>[4x]MSQNQVPKWIQLNNEIMIQKDGKFQFDKDKEAVHSYFVDYINQNTVFFHNLKEKLDYLVENQYYEEEFLSLYSFEDIKEVFKTAYAKKFRFPSFMSAFKFYNDYALKTNDKKKILERYEDRISIVALFFANGDTEKAKEYVNLMINQEYQPSTPTFLNAGRKRRGEL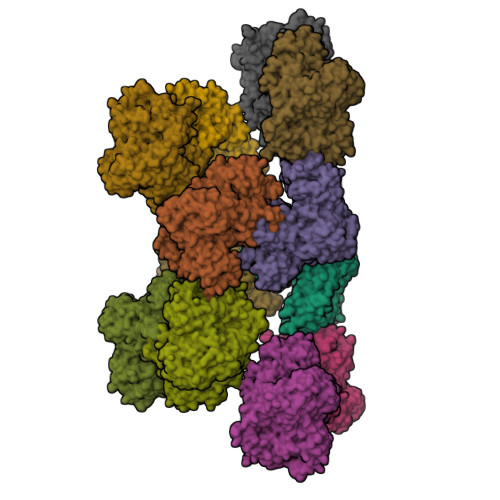VSCFLLEVNDSLNDISRAIDISMQLSKLGGGVSLNLSKLRAKGEAIKDVENATKGVVGVMKLLDNAFRYADQMGQRQGSGAAYLNIFHRDINDFLDTKKISADEDVRVKTLSIGVVIPDKFVELAREDKAAYVFYPHTIYKEYGQHMDEMDMNEMYDKFVDNPRVKKEKINPRKLLEKLAMLRSESGYPYIMFQDNVNKVHANNHISKVKFSNLCSEVLQASQVSSYTDYDEEDEIGLDISCNLGSLNILNVMEHKSIEKTVKLATDSLTHVSETTDIRNAPAVRRANKAMKSIGLGAMNLHGYLAQNGIAYESPEARDFANTFFMMVNFYSIQRSAEIAKEKGETFDQYEGSTYATGEYFDKYVSTDFSPKYEKIANLFEGMHIPTTEDWKKLKAFVAEHGMYHSYRLCIAPTGSISYVQSSTASVMPIMERIEERTYGNSKTYYPMPGLASNNWFFYKEAYDMDMFKVVDMIATIQQHIDQGISFTLFLKDTMTTRDLNRIDLYAHHRGIKTIYYARTKDTGQDSCLSCVV> MADVAGTSNRDFAGREQRLFNSEQYNYNNSLNGEVSVWVYAYYSDGSVLVINKNSQYKVGISETFKALKEYRCGQHNDSYDECEVNQSIYYPNGGDAR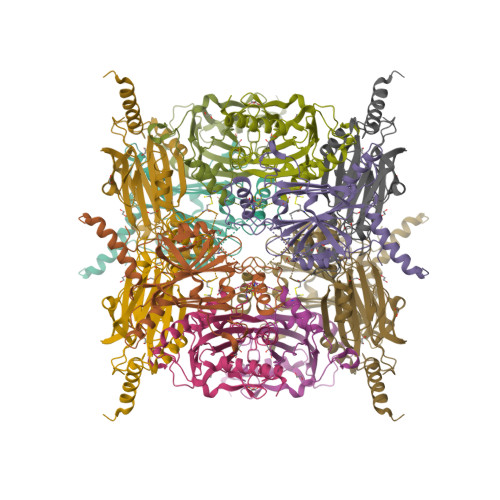KFHSNAKPRAIQIIFSPSVNVRTIKMAKGNAVSVPDEYLQRSHPWEATGIKYRKIKRDGEIVGYSHYFELPHEYNSISLAVSGVHKNPSSYNVGSAHNVMDVFQSCDLALRFCNRYWAELELVNHYISPNAYPYLDINNHSYGVALSNRQ>[2x]FSDTLEESSPIAAIFDTENLEKISITEGIERGIVDSITGQRLLEAQACTGGIIHPTTGQKLSLQDAVS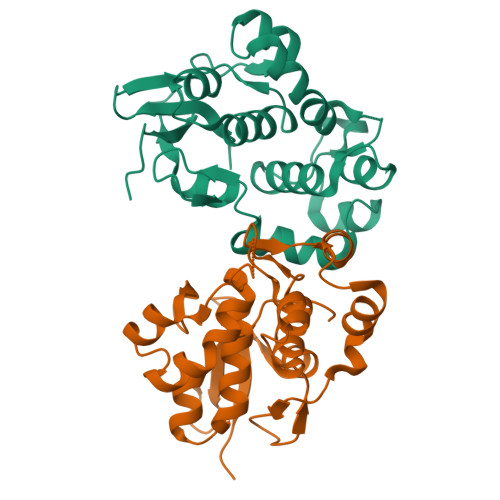QGVIDQDMATRLKPAQKAFIGFEGVKGKKKMSAAEAVKEKWLPYEAGQRFLEFQYLTGGLVDPEVHGRISTEEAIRKGFIDGRAAQRLQDTSSYAKILTCPKTKLKISYKDAINRSMVEDITGLRLLEAASVSSKGLPSPYNMSSA> MVPISPIETVPVKLKPGMDGPKVKQWPLTEEKIKALVEICTEMEKEGKISKIGPENPYNTPVFAIKKKDSTKWRKLVDFRELNKRTQDFWEVQLGIPHPAGLKKKKSVTVLDVGDAYFSVPLDEDFRKYTAFTIPSINNETPGIRYQYNVLPQGWKGSPAIFQSSMTKILEPFKKQNPDIVIYQYMDDLYVGSDLEIGQHRTKIEELRQHLLRWGLTTPDKKHQKEPPFLWMGYELHPDKWTVQPIVLPEKDSWTVNDICKLVGKLNWASQIYPGIKVRQLSKLLRGTKALTEVIPLTEEAELELAENREILKEPVHGVYYDPSKDLIAEIQKQGQGQWTYQIYQEPFKNLKTGKYARMRGAHTNDVKQLTEAVQKITTESIVIWGKTPKFKLPIQKETWETWWTEYWQATWIPEWEFVNTPPLVKLWYQLEKEPIVGAETFYVDGAANRETKLGKAGYVTNKGRQKVVPLTNTTNQKTQLQAIYLALQDSGLEVNIVTDSQYALGIIQAQPDKSESELVNQIIEQLIKKEKVYLAWVPAHKGIGGNEQVDKLVSAGIRKIL;> MVPISPIETVPVKLKPGMDGPKVKQWPLTEEKIKALVEICTEMEKEGKISKIGPENPYNTPVFAIKKKDSTKWRKLVDFRELNKRTQDFWEVQLGIPHPAGLKKKKSVTVLDVGDAYFSVPLDEDFRKYTAFTIPSINNETPGIRYQYNVLPQGWKGSPAIFQSSMTKILEPFKKQNPDIVIYQYMDDLYVGSDLEIGQHRTKIEELRQHLLRWGLTTPDKKHQKEPPFLWMGYELHPDKWTVQPIVLPEKDSWTVNDIQKLVGKLNWASQIYPGIKVRQLSKLLRGTKALTEVIPLTEEAELELAENREILKEPVHGVYYDPSKDLIAEIQKQGQGQWTYQIYQEPFKNLKTGKYARMRGAHTNDVKQLTEAVQKITTESIVIWGKTPKFKLPIQKETWETWWTEYWQATWIPEWEFVNTPPLVKLWYQLEKEPIVGAETF

A packaged viral enzyme, reverse transcriptase (RT), initiates DNA synthesis at the 3′-end of a host tRNALys3 that is part of a binary complex preassembled with the 5′-end of the HIV-1 viral RNA, called the primer-binding site (PBS). Kinetic investigations have shown that reverse transcription initiation on this vRNA–tRNALys3 template–primer complex is slow (~500-fold slower than elongation), nonprocessive, and displays a distinct pausing pattern along with the viral genomic RNA (vRNA) template. The resulting minimal vRNA–tRNA template–primer complex contained a 26-nucleotide fragment of the vRNA genome and a 39-nucleotide truncated tRNALys3. To circumvent the rapid dissociation of RT from dsRNA substrates, we adapted the previously employed disulfide cross-linking system to covalently link the RT p66 thumb domain to the vRNA–tRNA template–primer complex.

Using a minimal, active RNA initiation complex that spans the portions of vRNA and tRNA that reside within the RT cleft, while eliminating dynamic peripheral RNA elements that do not interact with the protein, we solved the structure of the minimal RT–vRNA–tRNALys3 initiation complex (miniRTIC) to 2.8-Å resolution, allowing for de novo modeling and definition of RT–RNA contacts. Density corresponding to the cross-link between p66 C258 and tRNA G71 is visible along the minor groove of the PBS helix. The miniRTIC, despite displaying activity in vitro, is captured in an inactive state unsuitable for nucleotide incorporation, as previously observed in lower-resolution studies of the initiation complex. The tRNA 3′ primer terminus is displaced ~5 Å from the canonical elongation primer site (P-site), away from the catalytic triad (D110, D185, and D186), and resides in the P′-site. This displacement is accompanied by an ~3-Å shift of the primer grip toward the thumb and away from the polymerase-active-site residues. In addition, the p66 thumb opens by ~6 Å and adopts a hyperextended conformation reminiscent of RT–DNA–NNRTI structures as reported in past analyses of lower-resolution RTIC structures. The tip of the fingers also hyperextends by ~5 Å to facilitate binding to the wide A-form vRNA–tRNA template–primer complex. The majority of protein–RNA contacts within the RTIC are located in two distinct regions that are one turn apart along the minor groove of the PBS helix. In our structures of early initiation, the RTIC features a sparse protein–nucleic acid contact landscape that likely underlies the poor affinity of RT for the vRNA–tRNALys3 template–primer complex.> MPELKVAFNKDTYVATVLDASGSVPSGSVNVGTFFHPDETYPDSYVIYHGVRELLYKRSEVDPAQPGFWPENITNMQAVTIDNKATARLVLNTSLPRVVSTIEGGKVTLSVVALGGKAPLKYKWEFRAPNAST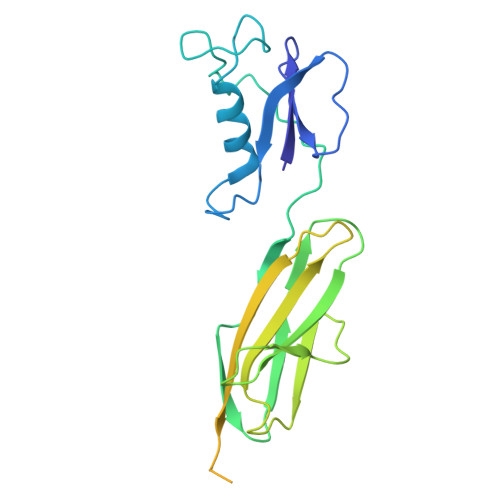WTAVSGQTTANLVLDNIDADKAGEYKVTVTDAAGTSVDSTALVAVGAYPPPALTGIKATPTSLSLSVATDAAGKTVALSAIPTDAELGTLSIKTAPDSARATATISGSTLTVKPVAAGAATSVVVTNGKVDVTITINVAA2-[[7-[4-(3,5-dimethylphenyl)carbonyl-2,6-dimethyl-phenoxy]-1-ethoxy-4-oxidanyl-isoquinolin-3-yl]carbonylamino]ethanoic acid | C31 H30 N2 O7 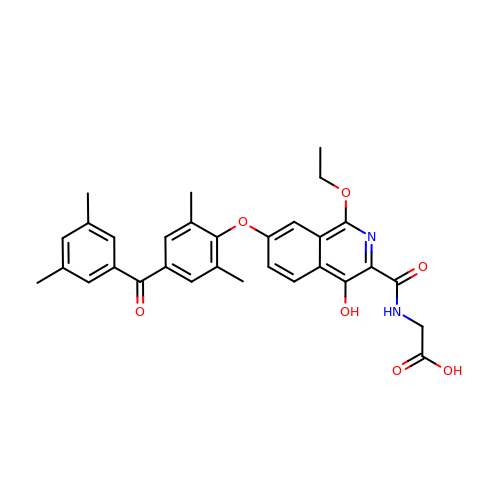| UXSXEVSQLAGZML-UHFFFAOYSA-N>HTPVRTVMNTIQQLMMILNSASDQPSENLISYFNNCTVNPKESILKRVKDIGYIFKEKFAKAVGQGCVEIGSQRYKLGVRLYYRVMESMLKSEEERLSIQNFSKLLNDNIFHMSLLACALEVVMATYSRSTSQNLDSGTDLSFPWILNVLNLKAFDFYKVIESFIKAEGNLTREMIKHLERCEHRIMESLAWLSDSPLFDLIKQSKDREGPTDHLESA[4x];>FQTQKPLKSTSLSLFYKKVYRLAYLRLNTLCERLLSEHPELEHIIWTLFQHTLQNEYELMRDRHLDQIMMCSMYGICKVKNIDLKFKIIVTAYKDLPHAVQETFKRVLIKEEEYDSIIVFYNSVFMQRLKTNI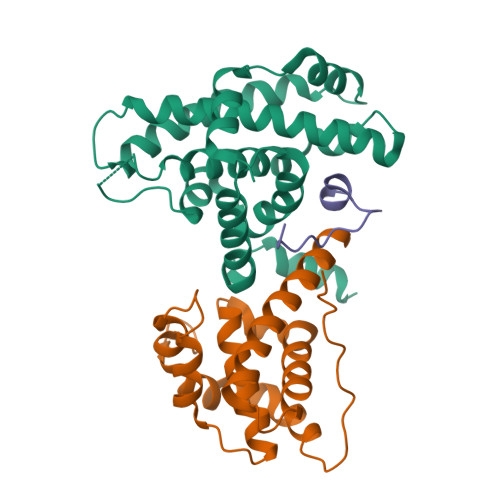LQYASTRPPTLSPIPHIPR[4x];>[4x]LDYHFGLEEGEGIRDLFD> MKLDIKKTFSNRSDRVKGIDFHPTEPWVLTTLYSGRVEIWNYETQVEVRSIQVTETPVRAGKFIARKNWIIVGSDDFRIRVFNYNTGEKVVDFEAHPDYIRSIA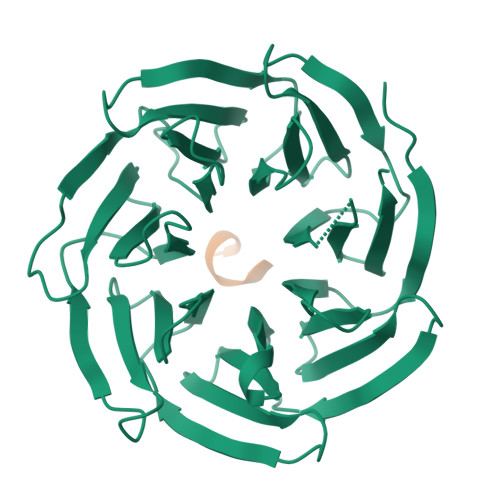VHPTKPYVLSGSDDLTVKLWNWENNWALEQTFEGHEHFVMCVAFNPKDPSTFASGCLDRTVKVWSLGQSTPNFTLTTGQERGVNYVDYYPLPDKPYMITASDDLTIKIWDYQTKSCVATLEGHMSNVSFAVFHPTLPIIISGSEDGTLKIWNSSTYKVEKTLNVGLERSWCIATHPTGRKNYIASGFDNGFTVLSLG;> FEAKKLV~{N}-(1,3,5-trimethylpyrazol-4-yl)methanesulfonamide 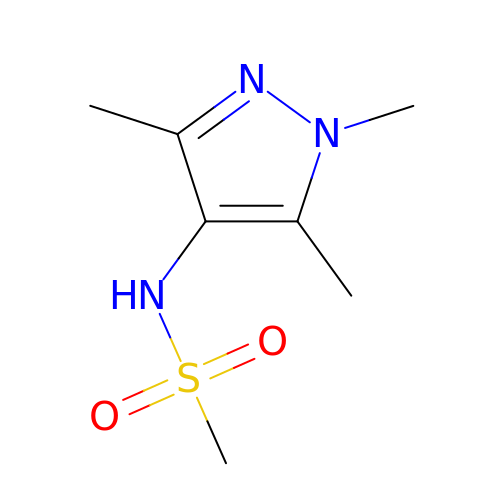| C7 H13 N3 O2 S | PADGNQOKIIWYMD-UHFFFAOYSA-N>[2x]MADEIAKAQVARPGGDTIFGKIIRKEIPAKIIFEDDRCLAFHDISPQAPTHFL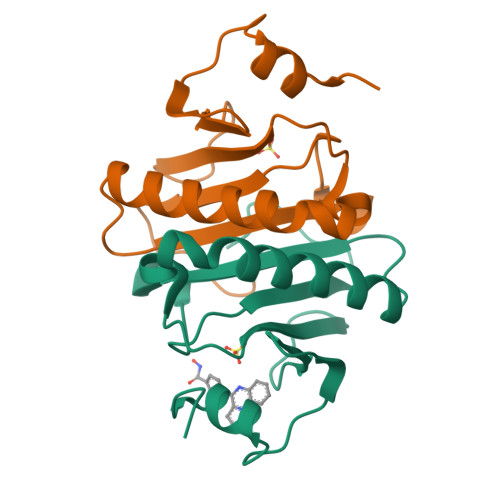VIPKKHISQISVAEDDDESLLGHLMIVGKKCAADLGLNKGYRMVVNEGSDGGQSVYHVHLHVLGGRQMHWPPG>MSSKAPKKSKQRSQPRNRTPNTSVKTVAIPFAKTQIIKTVNPPPKPARGILHTQLVMSVVGSVQMRTNNGKSNQRFRLNPSNPALFPTLAYEAANYDMYRLKKLTLRYVPLVTVQNSGRVAMIWDPDSQDSAPQSRQEISAYSRSVSTAVYEKCSLTIPADNQWRFVADNTTVDRKL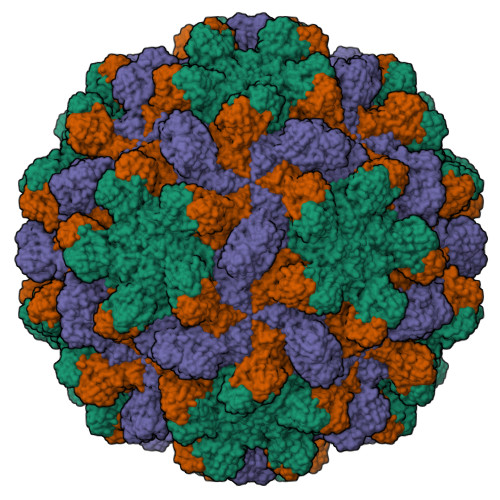VDFGQLLFVTHSGSDGIETGDIFLDCEVEFKGPQPTASIVQKTVIDLGGTLTSFEGPSYLMPPDAFITSSSFGLFVDVAGTYLLTLVVTCSTTGSVTVGGNSTLVGDGRAAYGSSNYIASIVFTSSGVLSTTPSVQFSGSSGVSRVQMNICRCKQGNTFILG[3x]> GPHMSAPNPKAFPLADAALTQQILDVVQQAANLRQLKKGANEATKTLNRGISEFIIMAADCEPIEILLHLPLLCEDKNVPYVFVPSRVALGRAC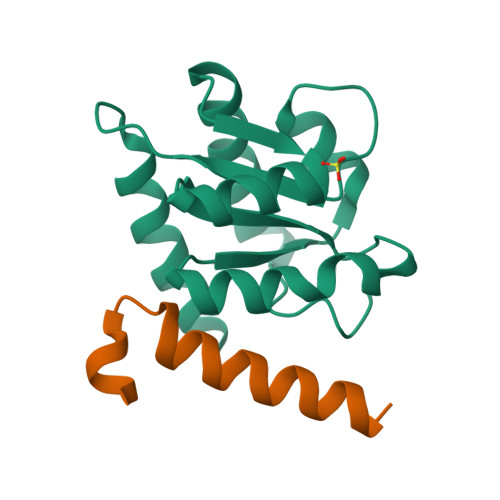GVSRPVIAASITTNDASAIKTQIYAVKDKIETLLI;> GPHMTDEDVKKWREERKKMWLLKISNNKQKHMQEMGIKEDELKSQPSIFKESRKEKQ>MSASTQHRAHRWPQPLPGNDRKIWFGADYNPDQWPEDVQDEDIRLMKQAGVNIVSLAIFSWANIETSDGNFEFDWLDRVIDKLYKAGIAVDLASATASPPMWLTSAHPEVLRRDEQGHVIWPGARQHWRPTSPTFRTYALRLCREMAEHYKDNPAIVSWHVGNEYGCHN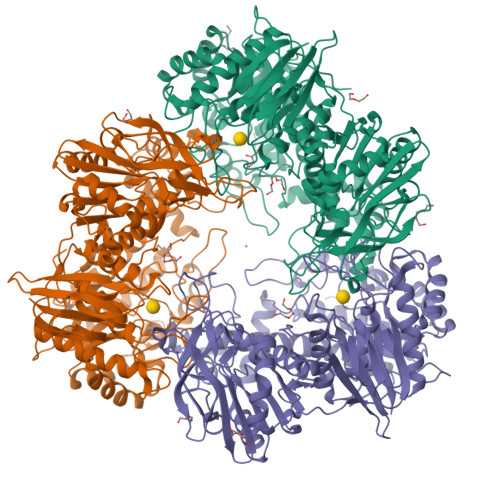YFDYSDDAVQAFREWCRDRYGTIDKVNAAWGTNFWSQRLNSFEEILPPRYVGGEGNFTNPGRLLDFKHFCSDALKEFFCAERDVLSEVTPNIPLTTNFMVSASQNTLDYDDWAHEVDFVSNDHYFTPGSWHIDELAYSASLVDGISRKKPWFLMEQSTSAVNWREINPRKEPGELIRDSMLHLAMGADAICYFQWRQSRSGAEKFHSAMLPLAGEHSQIYRDVCALGADLDTLSDAGILRSKLSKARVAIVQDIQSEWATEHTATPTQHIREWTEPLDWFAAFANRGVTADVTPIHAQWDTYDAVVIPCVYLFSEEMAERLRTFVRNGGKAFVTYYSALADEHDRLHTEGWPGLIGDVVGVRIEEHCPLGTLFPGMLDHLDVSNGTVVHDLADVIDAIADDTTVLATFEADPATGMDGRAAITVHPYHEGGVAYIAGKLGRDGISQSLPEICAALGFELDADPRAGDVLRVVREQEDGAIFEFLFNRTRNTVTADRPAGDMLICSLATDSTDKVTLEPNGVLAFRR[3x]>[30x]MAFEENLYCDYTPGAAKAVAGKDVILAVFNAAGDKLLAVAGQQGLTVNRSKDSIEITSKDTVGGWKSKIGGMKEWSIENDGLYVADAESHKELAKYFESDSPVCVKIINQASKKGLFGGLAIVADYSFEAPFDEA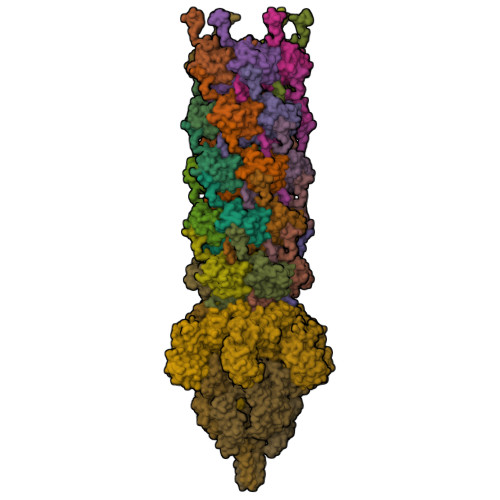MTYSVKLDGMGALVDLTITEGGDQMPGETPVAPAE;>[3x]MAESKSITFELNESVLTAQVGRLDEMAMVVERRFSELKMTIEDVGNADPGSKISESLGGLQSGLGTISSAFGQLGSSSEAITSGFGTAVGSVGGITDAFKNLGSSVQNGTLFSSLATGIGGMSTMLGGVSGGVQGITNLASGFMELKNHLGGLMSSIGGVGGIMGKLTSPMGLVIIGIVALVAAFTYLMTTNESFRNTVMSVVTQVAQLFGQLVASLMPIIMQIVTAVMQIGAALMPMVMQFISFFAQLLAQLMPFINMLISMLMPVIMQIVQVVMSLVSALLPSIMTVIQGIMSVIQFLIPIIMQIATVVVQIVVTIISYISKIMPIVMTIIGVIVSIITTIISYVVIIATTIASVIGKIISFIASVITAVIGIVQPIIAFITNIFTTIVTIIGAAFQMVFTVASKIWNSIMSTISGIIDGIKAVITGISTTVSSVFNGVKRIITGVFDGIKSAWGGLTDFVGNIFDGVSSAIQTVVDNVKGFVNVVIRGINGAIGLINKIPGVEIGKIPQLISGTTNFQGGFARMNEGGRGEMVVLPSGSQVIPHDATMKYARESARGNKSMLYTSQGADLARVENLLERLLQKNPVIKMDDKVVAEVVSRNQANSFDQYNYTMGGAAYS;>MSDLFLELNGKVHSLSETFPGLSVQEVSRQSPQLSMETAEIAGTDGVIPGMTQFKPFIFSAKCNLQALDIPDYHLAVREIYEFLFQRDSYYIWSDQMPGIRYEVHPKPVDFSRESDRVGLLTIEFDVFKGYAESRGTSLDPMTFEVDLWQMGMNLSNRDDLFYVFRENTFRVYNAGSDRVNPLMRHELDIAMTANGTPTIHNLTTGESFEYRKELQKTDVLLLNNIYPLVNNRRVGKDTNHGIITLEKGWNDFEIKGVTDVTIAFNFPFIYR[6x];>[3x]MDYVIIQSMDKEVEEILTDIDYGSFSYDYEKNTSRAISFTVNKTKQNAAIFDLVGNEAILTYQGQQFVIKKCTPKSIGGTISKQITAQHICYTVQDHVQYNVKSGRKKYSIQTVLEFALQDNVLGFSYEIQGSFPLVELEDLGNKNGLELVNLCLEEFGAILFADNKKLYFYDEKSWYVRTEKQFRYLYNTEEVSVDTNTDNLKTEIKCYGKQKENADKLTGDNKYMAVVTYTSPNEAIYGKRMANAKSDDKITNNDDLLIFAKKQILDVPETALTIAYKGKEPVSERDVWYFIHEPMGFETEVKVTKIKSSHPWSKKFQEIGFSNSRRDMVRIQTQIANQVKKASVDTNKINSFSSIAMNAYDSRILTEVVGVVDGD;>[3x]MATEIRVLKNVDDTVFYPKTHVTAVEGLDSATTTTSGLMPASDKTKLNGIEANAEKNNVTAIDIANWNKKQDAILVSENGSNFKITVTNAGELKATKVE2-(3,6-DIHYDROXYPHENYL)ACETIC ACID 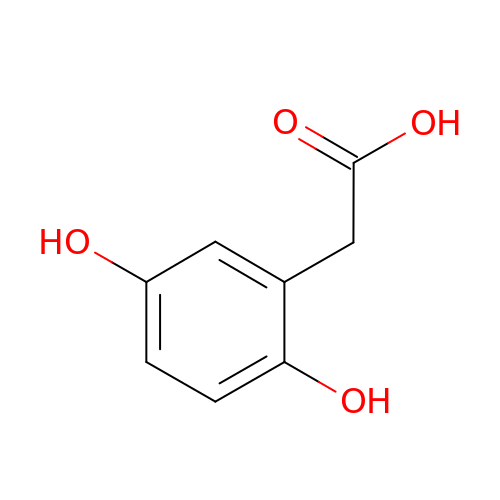| C8 H8 O4 | IGMNYECMUMZDDF-UHFFFAOYSA-N> HHHHHHMPSRTALSPGVLSPTRPVPNWIARPEYVGKPAAQEGSEPWVQT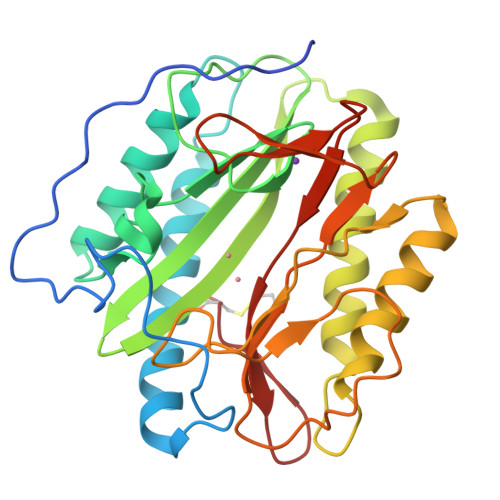PEVIEKMRVAGRIAAGALAEAGKAVAPGVTTDELDRIAHEYLVDNGAYPSTLGYKGFPKSCSTSLNEVICHGIPDSTVITDGDIVNIDVTAYIGGVHGDTNATFPAGDVADEHRLLVDRTREATMRAINTVKPGRALSVIGRVIESYANRFGYNVVRDFTGHGIGTTFHNGLVVLHYDQPAVETIMQPGMTFTIEPMINLGALDYEIWDDGWTVVTKDRKWTAQFEHTLLVTDTGVEILTCL> MATVLSPNQNNNSGSIPTGYSDLEFSLANGNWVKNLSLPTNANNSDKITIRSSAAYSSYLDTSNTNIPLEVLKINSGDVYQFIFNSSQNKWIAQLATVSPTTGSNYELIPLTTATMQKVLIQDDKWAQTIALPSDVRDGTTVQVVSTASVSSDIDKTNLLFPSSFTLKNGSEYWFKYYSALGKWVPEYIKPQKLNVQQIGTSLAAVNSPLTEIAFGDGNWVSNFTLPTTANDRDRIIIKSTATWSAKINNTNVNSQATLTLKTGDQYEFMYVSDKGYWQLISSPTKVIDSTATIPAILPNMTQPTLKVKLSTSNWQPTLQLPAQAQVGDKVVIVSNASADTYINAANGLSTAIKNGENRRFIYTAQGWTVDSYTIDMLLVSSPEVNSIL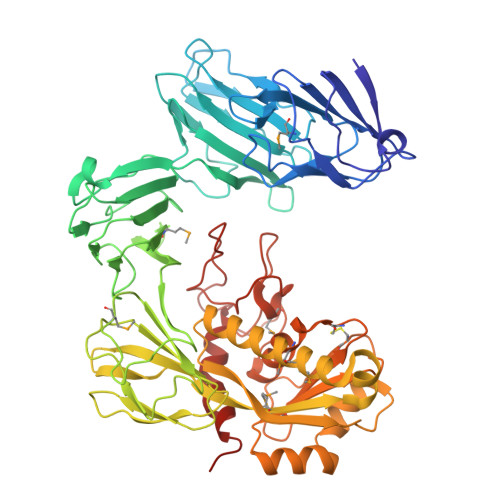GESAAKLRMIEGVNLTNLTAENSNARFYLRDVGYITYKIPAATLKEAISTGRDDTTVQNERKRILADGVYYQGNEPGDGGCGWAWINASAYNMIGANDIAGCSFAAMRHEVGHNLGLYHNGSTNIGSGFAHPLGSTAMGGNNINFYSSPYLYNPKYGVRLGEEGKIDAVSVINLNAQKISLYNHHHHHH> MSAEKLFTPLKVGAVTAPNRVFMAPLTRLRSIEPGDIPTPLMGEYYRQRASAGLIISEATQISAQAKGYAGAPGLHSPEQIAAWKKITAGVHAEDGRIAVQLWHTGRISHSSIQPGGQAPVSASALNANTRTSLRDENGNAIRVDTTTPRALELDEIPGIVNDFRQAVANAREAGFDLVELNSAHGYLLHQFLSPSSNQRTDQYGGSVENRARLVLEVVDAVCNEWSADRIGIRVS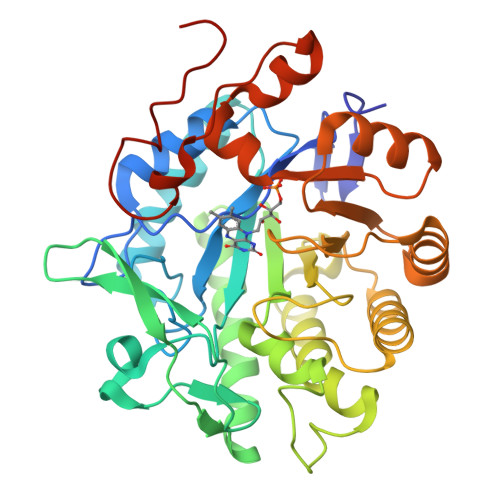PIGTFQNVDNGPNEEADALYLIEELAKRGIAYLHMSETDLAGGKPYSEAFRQKVRERFHGVIIGAGAYTAEKAEDLIGKGLIDAVAFGRDYIANPDLVARLQKKAELNPQRPESFYGGGAEGYTDYPSLHHHHHHHH>[2x]MYKVKVYVSLKESVLDPQ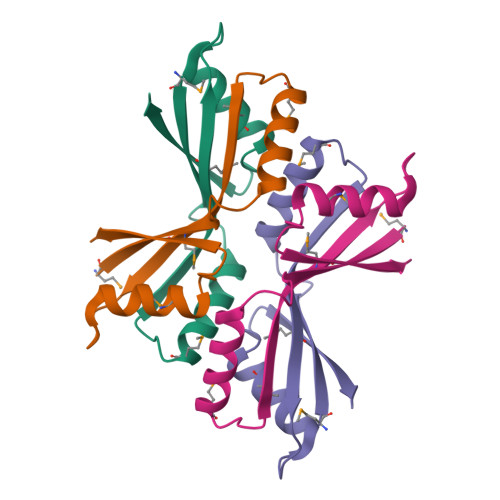GSAVQHALHSMTYNEVQDVRIGKYMELTIEKSDRDLDVLVKEMCEKLLANTVIEDYRYEVEEVVAQ>MLSPKAATLAERSAGLAFSLYQAMAKDQAVENILLSPVVVASSLGLVSLGGKATTASQAKAVLSAEQLRDEEVHAGLGELLRSLSNSTARNVTWKLGSRLYGPSSVSFAEDFVRSSKQHYNCEHSKINFRDKRSALQSINEWAAQTTDGKLPEVTKDVERTDGALLVNAMFFKPHWDEKFHHKMVDNRGFMVTRSYTVGVTMMHRTGLYNYYDDEKEKLQIVEMPLAHKLSSLIILMPHHVEPLERLEKLLTKEQLKIWMGKMQKKAVAISLPKGVVEVTHDLQKHLAGLGLTEAIDKNKADLSRMSGKKDLYLASVFHATAFEWDTEGNPFDQDIYGREELRSPKLFYADHPFIFLVRDTQSGSLLFIGRLVRPKGDKMRDELLEHHHHHH[2x];>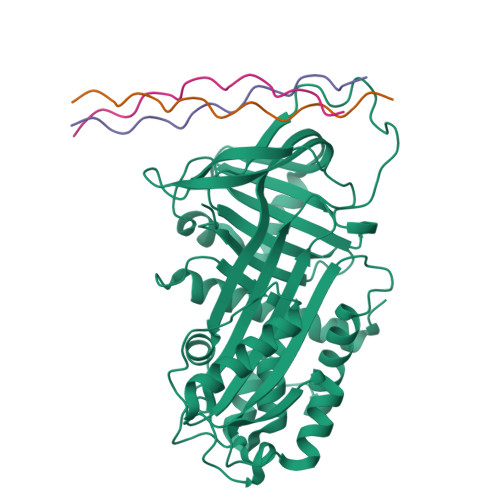[6x]XPPGPPGPPGPRGFPGPPGPPG>[2x]MHHHHHHGGLVPRGSHMKIGIIGAMEEEVTLLRDKIDNRQTITLGGCEIYTGQLNGTEVA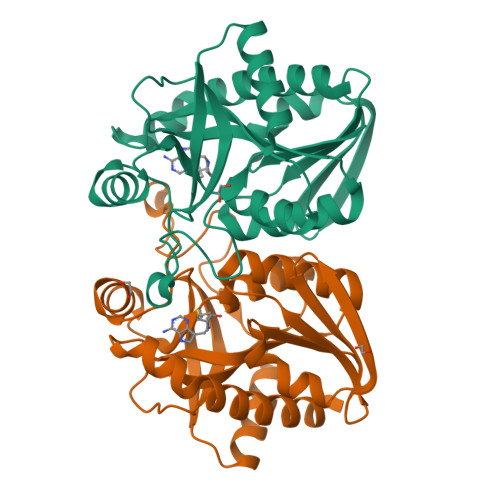LLKSGIGKVAAALGATLLLEHCKPDVIINTGSAGGLASTLKVGDIVVSDETRYHDADVTAFGYEYGQLPGCPAGFKADDKLIAAAESCIRELNLNAVRGLIVSGDAFINGSVGLAKIRHNFPDAVAVEMEATAIAHVCHNFNVPFVVVRAISDVADQQSHLSFDEFLAVAAKQSTLMVETLVQKLAHG> EDVVWRWSCDNGKCVKLKNDPRSSEPALSLEACKMFCNEYGLLWPRPTGEADLGNFLSKINLNSIEVKILKKGATDDLMEAAAKRFKEQVSLAIPRGSTPKLTGKAVDVYLVNENPNEKAFSLEMDESYGLRVSPSGADRVNATITANSFFGMRHGLETLSQLFVFDDIRDHLLMVRDVNISDKPVYPYRGILLDTARNYYSIESIKRTIEAMAAVKLNTNHWHITDSQSFPFVTTKRPNLYKFGALSPQKVYTKAAIREVVRFGLERGVRVLPEFDAPAHVGEGWQDTDLTVCFKAEPWKSYCVAPPCGQLNPTKDELYQYLEDIYSDMAEVFDTTDIFHMGGDEVSEACWNSSDSIQNFMMQNRWDLDKESFLKLWNYFQQKAQDKAYKAFGKKLPLILWTSTLTNYKHIDDYLNKDDYIIQVWTTGVDPQIKGLLEKGYRLIMSNYDALYFDCGYGAWVGAGNNWCSPYIGWQKVYDNSPAVIALEHRDQVLGGEAALWSEQSDTSTLDGRLWPRAAALAERLWAEPATSWQDAEYRMLHIRERFVRMGIQAESLQPEWCYQNEGYCYS

Insect OfHex1 from the Asian corn borer (Ostrinia furnacalis) is a β-N-acetyl-D-hexosaminidase specialized for chitin degradation during molting and metamorphosis. OfHex1 shows high activity toward β-1,4-linked chitooligosaccharides but is not able to hydrolyse β-1,2-linked GlcNAc from N-glycans, thus exhibiting very high substrate specificity. According to the CAZy database, β-N-acetyl-D-hexosaminidase belongs to family 20, and uses a substrate-assisted double displacement mechanism by which the 2-acetamido group in the substrate GlcNAc, instead of the acidic residue in a β-glucosidase, acts as the nucleophile. OfHex1 also contains a -1 subsite and +1 subsite for sugar moiety binding, and the three corresponding amino acid residues found in BGlu1 for binding the +1 GlcNAc are found in OfHex1(Val327, Glu328 and Trp490).

Since we have obtained the structure of OfHex1 V327G mutant previously, in this study, the crystallization of E328A in complex with TMG-chitotriomycin was performed and the complex structure was resolved to 2.5 Å. According to the alignment, the mutation of Glu328 to Ala resulted in obvious conformation changes. The catalytic residues, Glu368 and Asp367 are rotated about 180° and 90° compared to those in the OfHex1-TMG-chitotriomycin complex but with similar conformations as those in the apo-structure of OfHex1. The rotation of Glu368 led to the collapse of the two important hydrogen bond networks (Asp249-His303-Glu368 and Glu328-H2O (I)-Glu368). In addition, the mutation of Glu328 to Ala increased the volume of the active pocket from 646.8 Å3 to 758.3 Å3 as measured with CASTp, suggesting an important role of Glu328 in constructing the active pocket. The conformation of TMG-chitotriomycin, in particular the GlcNAcII moiety, was found to be very different from that observed in the wild-type. The most obvious change is the absence of short polar interaction between Glu328 and the C3-OH of GlcNAcI of TMG-chitotriomycin. Interestingly, a water molecule was found to occupy the position of the side chain of Glu328. The interaction between the nitrogen atom of the 2-acetamido group (GlcNAcII) and the oxygen atom of the carbonyl group (main chain of Trp490) is missing, but instead, C6-OH of GlcNAcII forms a hydrogen bond with the main chain of Val327. Site-directed mutagenesis indicated the change of Glu328 to Ala impaired OfHex1’s affinity toward the substrate, (GlcNAc), by 8-fold and the inhibitory activity of TMG-chitotriomycin by 42-fold.> MAILTDENYVDKAERAISLLEKDNKGNYLLTTSQIRKLLSLCSSLYDRSKERKFDELINDVSYLRVQFVYQAGREIAVK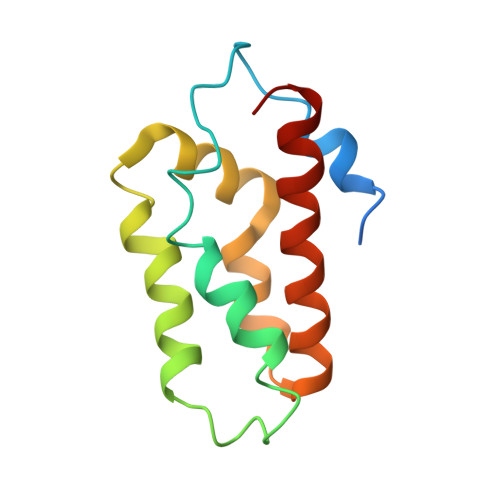DLIEKAQILEALKEIKDRETLQRFCRYMEALVAYFKFYGGKD> SESNKAGEDGASTVERETQEDDTNSIDSSDDLDGFVKILKEIVKLDNIVSSTWNPLDESILAYGEKNSVARLARIVETDQEGKKYWKLTIIAELRHPFALSASSGK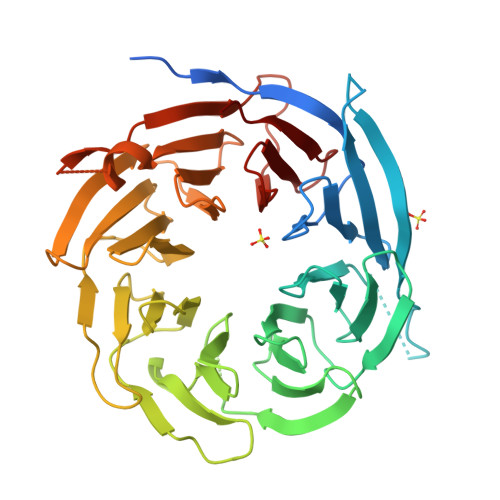TTNQVTCLAWSHDGNSIVTGVENGELRLWNKTGALLNVLNFHRAPIVSVKWNKDGTHIISMDVENVTILWNVISGTVMQHFELKETGGSSINAENHSGDGSLGVDVEWVDDDKFVIPGPKGAIFVYQITEKTPTGKLIGHHGPISVLEFNDTNKLLLSASDDGTLRIWHGGNGNSQNCFYGHSQSIVSASWVGDDKVISCSMDGSVRLWSLKQNTLLALSIVDGVPIFAGRISQDGQKYAVAFMDGQVNVYDLKKLNSKSRSLYGNRDGILNPLPIPLYASYQSSQDNDYIFDLSWNCAGNKISVAYSLQEGSVVAIPG Integrins are heterodimeric transmembrane receptors composed of alpha (α) and beta (β) subunits that link extracellular ligands to the actin cytoskeleton through intracellular adaptors. Cytoplasmic adapter proteins including KINDLIN2, Integrin-β1 binding protein 1 (ICAP1) and to a lesser extend FilaminA were shown to bind the Integrin-β1 peptide in the proximity of the K794-containing distal NPXY-motif. Integrin capture by the PH-domain-dependent membrane-associated KINDLIN2 is a key event in the induction of cell adhesion, even prior to TALIN1-association. Structural analysis of Integrin-β1 interaction with KINDLIN2, biochemical pulldown assay, and binding energy determination by using molecular dynamics simulation showed that acetylation of K794 and the K794Q-mutant increased KINDLIN2 binding affinity to the Integrin-β1.

We mutated the Lys794 to glutamine (Gln), an amino acid that was previously used to mimic acetylated Lys-residues of proteins as it provides charge neutralization and shares hydrogen-bonding capacities with the acetyl group. We also determined the crystal structures of Kindlin2 fused to the β1-K794Q peptide at 2.49 Å resolution. The surface representation of Kindlin2 indicated that the β1-K794Q peptide is bound closer to the Kindlin2 F3 subdomain than the wildtype β1 peptide, and that the β1-AcK794 peptide fits the Integrin binding groove of Kindlin2 more snugly than the wildtype peptide. (F) B-factor index for the respective B-factors of the wildtype and K794Q-mutant Integrin sequences demonstrating stabilization of the c-terminal KYEG-peptide sequence by the introduction of the acetyl-mimetic mutation (QYEG). Since B factors represent the atomic displacement and mobility of the side chain, this result further supports the notion that the K794Q mutation in β1 peptide enhances its binding with KINDLIN2. The peptide carrying the acetylation mimetic K794Q mutation also showed enhanced binding of KINDLIN2 compared to the non-modified peptide. but still had less negative dG than the peptide carrying the longer and positively charged arginine residue (K794R). Nonetheless, the biochemical affinity data validated the use of the K794Q mutation as a relevant model to recapitulate the effect of Integrin-β1 acetylation in cells. In the specific experimental case of permanent acetylation mimetism by the constitutive expression of the K794Q-mutant of Integrin-β1, KINDLIN2 is recruited with higher affinity leading to the formation of dysregulated immature adhesion.

>[2x]MALDGIRMPDGCYADGTWELSVHVTDLNRDVTLRVTGEVHIGGVMLKLVEKLDVKKDWSDHALWWEKKRTWLLKTHWTLDKCGIQADAKLQFTPQHKLLRLQLPNMKYVKVKVNFSDRVFKAVSDICKTFNIRHPEELSLLKKPRDPTKKKKKKLDDQSEDEALELEGPLIMPGSGSIYSSPGLYSKTMTPTYDAHDGSPLSPTSAWFGDSALSEGNPGILAVSQPVTSPEILAKMFKPQALLDKAKTNQGWLDSSRSLMEQDVKENEALLLRFKYYSFFDLNPKYDAIRINQLYEQAKWALLLEEIECTEEEMMMFAALQYHINKLSIMTSENHLTTDVNPECLVSPRYLKKYKSKQITARILEAHQNVAQMSLIEAKMRFIQAWQSLPEFGITHFIARFQGGKREELIGIAYNRLIRMDASTGDAIKTWRFSNMKQWNVNWEIKMVTVEFADEVRLSFICTEVDCKVVHEFIGGYIFLSTRAKDQNESLDEEMFYKLTSGWV;>KSAVTTVVNPQYEGK[2x]Paramyxovirus fusion is typically mediated by two glycoproteins on the surface of virions: a trimeric fusion protein, F, with type I viral fusion protein characteristics, and a receptor binding protein variously named HN, H, or G depending on the virus and protein functionality. HN proteins have at least three functions: (1) they bind sialic acid receptors on glycoproteins and gangliosides at the cell surface (hemagglutinin activity). (2) HN proteins are neuraminidases, which catalyze the hydrolysis of glycosidic linkages on terminal sialic acid residues thus destroying the receptor. (3) A function common to paramyxovirus attachment proteins is to lower the activation barrier of the F protein, presumably through direct interaction, thereby triggering a major refolding event in F from a metastable prefusion form to a highly stable post-fusion form.

Here, we report the structure of the PIV5 HN ectodomain (residues 61–565), which adopts a hybrid state compared to the previously observed 4-heads-down and 4-heads-up conformations. Upon optimizing conditions, HN crystallized in the I4 space group and diffracted X-rays to ∼2.5 angstroms. Two disulfide-linked heads are in the up position, while two are in the down position (2-heads-up/2-heads-down), and the structure exhibits a novel non-covalent DOD interface between one head in the up position and one head in the down position (hereafter, the DOD interfaces observed in the 4-heads-up and 2-heads-up/2-heads-down conformations will be referred to as DOD1 and DOD2, respectively). A stalk/head interface is indeed observed in the current structure, which resembles that of NDV HN in that covalently-linked heads are in the down position allowing one head to form a similarly sized interface with the stalk (buried solvent-accessible surface area = 1,294 and 1,185 Å2 for PIV5 and NDV using similar methods, respectively). Like the stalk/head interface in NDV HN, the PIV5 HN interface is primarily hydrophobic with 28 hydrophobic interactions and 5 electrostatic interactions including two hydrogen bonds and two salt bridges. The stalk of chain B extends beyond the 4HB core, which ends at residue L101, forming an extended alpha helix through N110. This extended helix also corresponds to the positioning of the head of this chain higher than its covalent partner and is consistent with the 4-heads-up conformation, where one head of each covalent dimer extends higher than its partner leading to a ∼30° offset between covalent dimers across the DOD1 interface. A novel dimer-of-dimers interface lacking pseudo-tetrameric symmetry is observed between one head of one disulfide-linked dimer in the up position (chain A) and another (chain D) in the down position (DOD2). This ∼2-fold symmetric interface buries ∼1,139 Å2 (total) of solvent-accessible surface area and includes 16–17 residues from each of the two heads.

>SPSSGLGSITDLLNNILSVANQIIYNSAVALPLQLDTLESTLLTAIKSLQTSDKLEQNCSWSAALINDNRYINGINQFYFSIAEGRNLTLGPLLNMPSFIPTATTPEGCTRIPSFSLTKTHWCYTHNVILNGCQDHVSSNQFVSMGIIEPTSAGFPFFRTLKTLYLSDGVNRKSCSISTVPGGCMMYCFVSTQPERDDYFSAAPPEQRIIIMYYNDTIVERIINPPGVLDVWATLNPGTGSGVYYLGWVLFPIYGGVIKGTSLWNNQANKYFIPQMVAALCSQNQATQVQNAKSSYYSSWFGNRMIQSGILACPLRQDLTNECLVLPFSNDQVLMGAEGRLYMYGDSVYYYQRSNSWWPMTMLYKVTITFTNGQPSAISAQNVPTQQVPRPGTGDCSATNRCPGFCLTGVYADAWLLTNPSSTSTFGSEATFTGSYLNTATQRINPTMYIANNTQIISSQQFGSSGQEAAYGHTTCFRDTGSVMVYCIYIIELSSSLLGQFQIVPFIRQVTLS[4x]N1-(4,5-dihydro-1H-imidazol-2-yl)-N4-(4-((4,5-dihydro-1H-imidazol-2-yl)amino)phenyl)benzene-1,4-diamine | C18 H21 N7 | 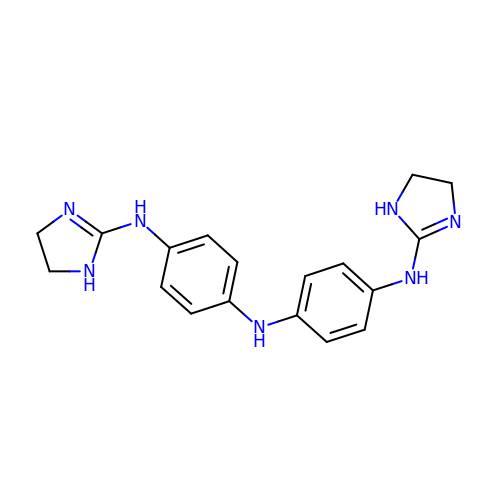AJWTXSLKVJNYAB-UHFFFAOYSA-N>[2x]MERTFVMIKPDGVQRGLIGEIISRFERKGFKIVAMKLMRISQELAEKHYAEHREKPFFSGLVDFITSGPVVAMVLEGKN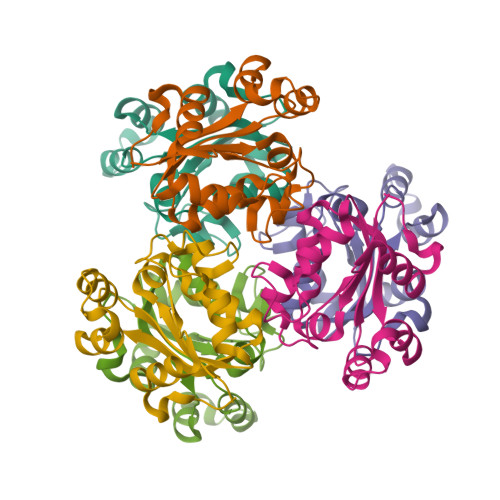VVEVVRKMIGATNPKEAAPGTIRGDFGMSVGKNVIHGSDSLESAEREISLFFKDEELVEW> MSQYSIQQSLGNASGVAVSPINADATLSTGVALNSSLWAGIGVFARGKPFTVLAVTESNYEDVLGEPLKPSSGSQFEPIRHVYEAIQQTSGYVVRAVPDDAKFPIIMFDESGEPAYSALPYGSEIELDSGEAFAIYVDDGDPCISPTRELTIETATADSAGNERFLLKLTQTTSLGVVTTLETHTVSLAEEAKDDMGRLCYLPTA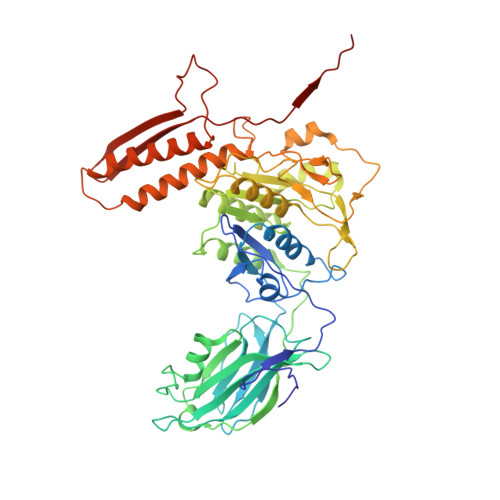LEARSKYLRAVVNEELISTAKVTNKKSLAFTGGTNGDQSKISTAAYLRAVKVLNNAPYMYTAVLGLGCYDNAAITALGKICADRLIDGFFDVKPTLTYAEALPAVEDTGLLGTDYVSCSVYHYPFSCKDKWTQSRVVFGLSGVAYAAKARGVKKNSDVGGWHYSPAGEERAVIARASIQPLYPEDTPDEEAMVKGRLNKVSVGTSGQMIIDDALTCCTQDNYLHFQHVPSLMNAISRFFVQLARQMKHSPDGITAAGLTKGMTKLLDRFVASGALVAPRDPDADGTEPYVLKVTQAEFDKWEVVWACCPTGVARRIQGVPLLIK> MHHHHHHMLRHNVPVRRDLDQIAADNGFDFHIIDNEIYWDESRAYRFTLRQIEEQIEKPTAELHQMCLEVVDRAVKDEEILTQLAIPPLYWDVIAESWRARDPSLYGRMDFAWCGNAPVKLLEYNADTPTSLYESAYFQWLWLEDARRSGIIPRDADQYNAIQERLISRFSELYSREPFYFCCCQDTDEDRSTVLYLQDCAQQAGQESRFIYIEDLGLGVGGVLTDLDDNVIQRAFKLYPLEWMMRDDNGPLLRKRREQWVEPLWKSILSNKGLMPLLWRFFPGHPNLLASWFDGEKPQIAAGESYVRKPIYSREGGNVTIF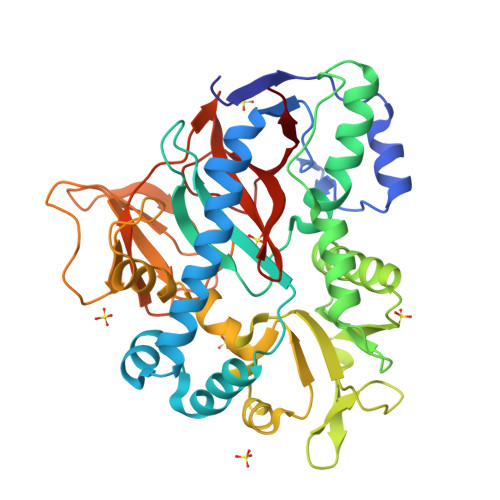DGKNNVVDHADGDYADEPMIYQAFQPLPRFGDSYTLIGSWIVDDEACGMGIREDNTLITKDTSRFVPHYIAG The assembly of about a 100 copies of a single protein, FlgE, makes the bacterial flagellar hook. The hook functions like a universal joint. It transmits the torque, produced by the motor located in the cell membrane, to the filament that acts like a propeller. Intriguingly, the C. jejuni hook protein, FlgEcj, has one of the longest amino acid sequences compared with other bacterial FlgE proteins.

We solved the structure of the hook of a fliK null mutant strain derived from C. jejuni strain 81116 (NCTC 11828) by electron cryo-microscopy, using single-particle averaging methods with image segment classification followed by systematic symmetry exploration. The final combined reconstruction yielded a map at 3.5 Å resolution that was used to build the model of FlgE. The structure of the hook protein of C. jejuni shows five distinct domains: D0, D1, D2, D3 and D4. The hook of C. jejuni is composed of 11 protofilaments that run along its length. The diameter of the hook is 280 Å, which is substantially wider than the hook of S. enterica that is 180 Å wide. In the hook, this central channel is made by the C-terminal α-helices from different protofilaments. These α-helices are closely packed and make the channel look like a continuous and smooth hollow structure with a diameter of 16 Å. The L-shaped stretch (L-stretch) [Gly32-Gln81] in domain D0 of FlgE is the segment of the hook structure that has the most contacts between the different FlgE molecules making the hook. The L-stretch is engulfed in a pocket surrounded by six molecules of FlgE that belong to four different protofilaments. However, the presence of domains D3 and D4 increase the number of interactions between the molecules of FlgE of C. jejuni, both within and between protofilaments.

> MRSLWSGVSGLQAHQVAMDVEGNNISNVNTTGFKYSRADFGTMFSQTVKIATAPTDGRGGSNPLQIGLGVSVSSTTRIHSQGSVQTTDKNTDVAINGDGFFMVSDDGGLTNYLTRSGDFKLDAYGNFVNNAGFVVQGWNINWDDQTIDSSRTPQNIFIDPGMHIPAAKSTEVAIKANLNSGLNIGTSSRNLYALDSVHGWNTKTQRAEDENDTGTTQFYTTSKNSVEVTEKGVDAGALFNANGTGLNLRDGQGIWVSYADAKFTTDRANGANVFDPNLTVAQQNNVIFWGNKDIAVTLDINLNGVRIQNDNIRSLDEAIAYINTFTAPTDTRDGTGVKAVKKADGSGIEFVNNNADGTTDNMKNIDLTVNVGNSAGERNTINYNANTGVFSPQGGNLTTAQNDTDWIAGAAQAGQPQNVKVVTAHKYIYSSNPVTIPPMINPDGGPAFQPNNGNRPTDPASANYWDAIQGSLKNTTERTFRTTEDLRELLQRDARYGVDYNGSGIIDNATPTFDANDINQAVKVVVTENGNFAISNANETSTIPANAGAGAGAATTNPKNMSFNITAYSNKQGTVSTNDAFTKIFKAFDGPLVIGNQIKESEQLKLSAFSAGLEIYDSLGSKHTLEVQFVKQSTTQDGGNEWQMIIRVPEPAEINTTGEGPTNIIVGTARFNNDGSLANYTPKTINFSPNNGAAPNQQIKLSFGTSGSNDGLVSSNSASTLTGQATDGYTSGNLKPDAIRVDDKGNILGEFTNGKTFAVAKIAMASVANNSGLEEIGGNLFKVTANSGNIVVGEAGTGGRGEMKTSALEMSNVDLSRSLTELIIIQRGYQANSKTISTSDQMLQTLIQLKQ>[8x]GSHSEADNYARELKREQEEII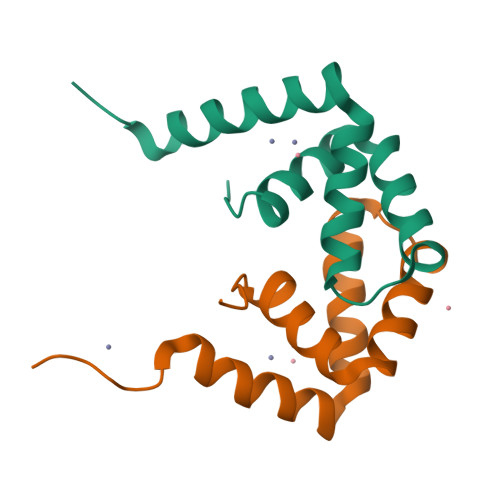RVPDTEAAEVAEILARYGIEPHEYGPVVNALRKKPQAWLDFMMKFELGLEKPDPKRAL>[2x]GSHMTVATDNNPTPEAVADLKKKVRKLNSKAGQM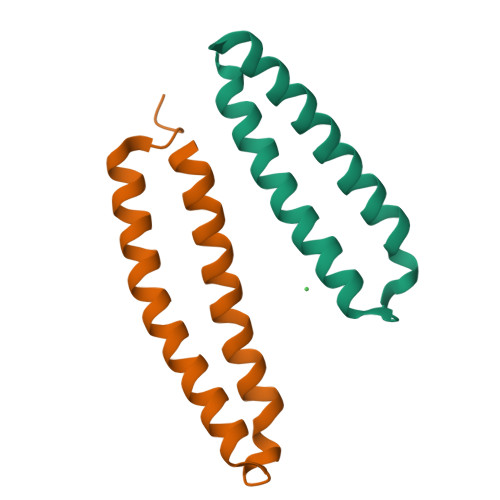KMDLHDLAEGLPTDYENLVETAEKTYEIFRELDQLKKKLNIWEETLK>ESSRSAMMYIQELRSGLRDMHLLSCLESLRVSLNNNPVSWVQTFGAEGLASLLDILKRLHDEKEETSGNYDSRNQHEIIRCLKAFMNNKFGIKTMLETEEGILLLVRAMDPAVPNMMIDAAKLLSALCILPQPEDMNERVLEAMTERAEMDEVERFQPLLDGLKSGTSIALKVGCLQLINALITPAEELDFRVHIRSELMRLGLHQVLQELREIENEDMKVQLCVFDEQGDEDFFDLKGRLDDIRMEMDDFGEVFQIILNTVKDSKAEPHFLSILQHLLLVRNDYEARPQYYKLIEECVSQIVLHKNGTDPDFKCRHLQIDIERLVD[4x];>KKVYKPEVQLRRPNWSKFVAEDLSQDCFWTKVKEDRFENNELFAKLTLAFSAQTKTSKAKKDQEGGEEKKSVQKKKVKELKVLDSKTAQNLSIFLGSFRMPYQEIKNVILEVNEAVLTESMIQNLIKQMPEPEQLKMLSELKEEYDDLAESEQFGVVMGTVPRLRPRLNAILFKLQFSEQVENIKPEIVSVTAACEELRKSENFSSLLELTLLVGNYMNAGSRNAGAFGFNISFLCKLRDTKSADQKMTLLHFLAELCENDHPEVLKFPDELAHVEKASRVSAENLQKSLDQMKKQIADVERDVQNFPAATDEKDKFVEKMTSFVKDAQEQYNKLRMMHSNMETLYKELGDYFVFDPKKLSVEEFFMDLHNFRNMFLQAVKENQKRRETEEKMRRAKLAKEKAEKERLEKQQKREQLIDMNAEGDETGVMDSLLEALQSGAAFRRKRGPRQVNRKAG[4x]

Formins are conserved actin regulators, which function in formation of stress fibers, actin cables, the cytokinetic ring and filopodia. Diaphanous-related formins (DRFs) including mDia, Daam and FRL are effectors of Rho family GTPases, which function in processes such as cell migration, cytokinesis, cell polarity signaling, phagocytosis, and cancer metastasis. In isolation, DRFs are autoinhibited through binding of a C-terminal diaphanous autoinhibitory domain (DAD), which immediately follows the FH2 domain in sequence, and an N-terminal diaphanous inhibitory domain (DID).

Here we report the crystal structure of an autoinhibitory complex of mDia1 formed in trans between the DID-DD and FH2-DAD fragments of the protein. Only the construct completely lacking the CC region (residues 131–457, DID-DD) yielded crystals in complex with FH2-DAD. These diffracted to 2.75 Å under synchrotron illumination. In the crystal, an asymmetric unit contains four chains each of DID-DD and FH2-DAD, consistent with the heavier mass observed in our ultracentrifugation and MALS data above. These are organized into two dimers of DID-DD (blue and grey in Fig. 2A), each of which is bound to a DAD element (red), and four bridge elements (dark/light green and dark/light tan). The linkers between bridge elements are not observed in the electron density, nor are the connections from bridge to DAD. In the autoinhibited structure presented here, the long axes of the DID elements are roughly collinear, with a relative angle of 167°, and the DD dimer is slightly displaced perpendicularly to this axis. The mDia1 lasso wraps around the post region as seen in Bni1p and Daam1, confirming a universal structure of the FH2 domain. At Leu1169 it connects to a loop that joins to the α-helical region of the DAD (Val1181-Gly1192), which is bound to the concave surface of the DID and ends at Phe1195. The weak electron density for the αT-DAD loop suggests that this element is flexible. The interaction between the DID and DAD is essentially the same as observed in the previously described DID•DAD and DID-DD•DAD complexes with backbone r.m.s.d. of 0.6 Å and 1.5 Å, respectively, between DAD on superimposed DIDs.The insulin-linked polymorphic region is a variable number of tandem repeats region of DNA in the promoter of the insulin gene that regulates transcription of insulin. This region is known to form the alternative DNA structures, i-motifs and G-quadruplexes. The C-rich sequence can form i-motif structures, comprised of two parallel stranded hairpins zipped together by intercalated, hemi-protonated cytosine-cytosine base-pairs. A crystal structure of an intramolecular i-motif also reveals that the sequences within the loop regions, and their additional stabilising interactions, are critical to formation of the stable i-motif structures.

With this in mind, we wanted to give the best chance for successful crystallisation, so we trialled the most stable C-rich ILPR variant that formed only i-motif from our biophysical studies: (4C) TATCCCCACACCCCTATCCCCACACCCCTAT. The crystallisations were performed at pH 5.5, below the pHT, where this sequence would be most stable. As there are two i-motifs in the asymmetric unit, this gives a view to how more than one i-motif may interact with each other like “beads-on-a-string”. Each of these individual i-motifs is formed from four antiparallel strands held together by eight, intercalated hemi-protonated cytosine-cytosine base pairs, connected by three loops. The ACA-loops connect strands at the minor grooves and the middle TAT-loop at the major groove. B Schematic showing the two 4C intramolecular i-motifs as arranged in the asymmetric unit and the interactions they form. Both fold into a 3′E-topology with the outer CC pair at the 3′–end (red). Apart from the CC-base-pairing, other interactions within each strand include mismatched base pairs like AA and TT, which could contribute to the overall stability of the folded construct. In strand-A, there is an AA base-pair between loop-1 and loop-3, A22 (loop-3) interacts with A10 (loop-1) via two hydrogen-bonds. Also, the flanking T3 interaction with T17 as a TT-base-pair stacks with the terminal CC-base-pair (C14 and C28). Given the potential binding pocket revealed by A16, which in strand-A is base-paired with T15 and in strand-B this adenine was displaced with a symmetry-related adenine, this indicates that this site may also be interesting for potential targeting with ligands.

>[2x]TATCCCCACACCCCTATCCCCACACCCCTAT>MIKIIIVAHGNFPDGILSSLELIAGHQEYVVGINFIAGMSSNDVRVALQREVIDFKEILVLTDLLGGTPFNVSSALS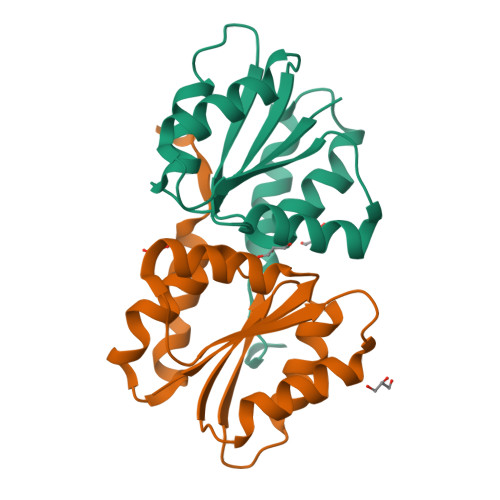VEYTDKKIKVLSGLNLSMLMEAVLSRTMFEHVDDLVDKVITSSHEGIVDFSTCLATQTAEATFEGGILEHHHHHH[6x]>[5x]GGMEVLDLVTGPDSVTEIEAFLNPRMGQPPTPESLTEGGQYYGWSRGINLATSDTEDSPGNNTLPTWSMAKLQLPMLNEDLTCDTLQMWEAVSVKTEVVGSGSLLDVHGFNKPTDTVNTKGISTPVEGSQYHVFAVGGEPLDLQGLVTDARTKYKEEGVVTIKTITKKDMVNKDQVLNPISKAKLDKDGMYPVEIWH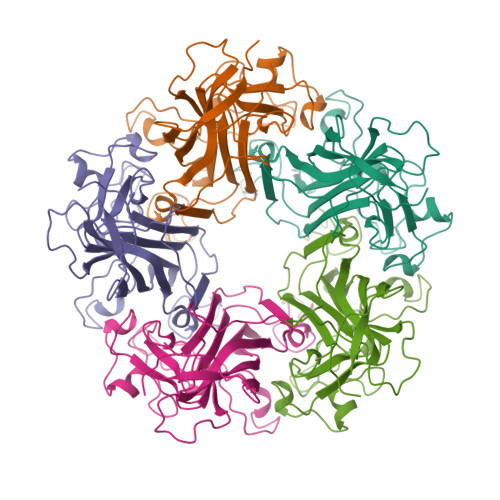PDPAKNENTRYFGNYTGGTTTPPVLQFTNTLTTVLLDENGVGPLCKGEGLYLSCVDIMGWRVTRNYDVHHWRGLPRYFKITLRKRWVKNPYP>APAIQILNFTFDKSVITN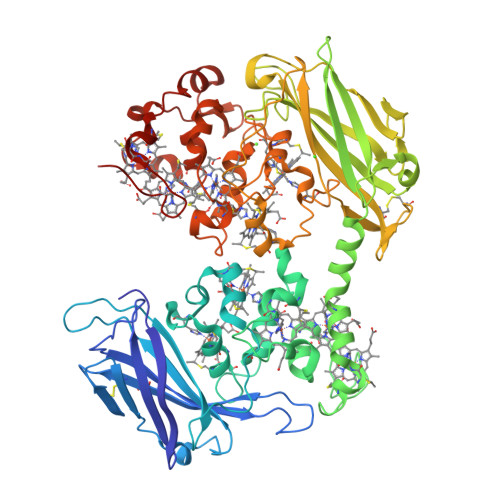GVPSVEFTVTNENDLPVVGLQKMRFAAAQLIPQGATGAGNASQWQYFGDETCDVAATCPGTFVDQKNGHYSYTFNMNLTANAKITYNDQLAQRVLIRAYNTPLPDGTQVPNSNAFVDFTADTGAAPTYSRKIVATESCNTCHQDLANVKHGGAYSDVNYCATCHTAGKVGVGKEFNVLVHAKHKDLTLGSLESCQSCHAANDAAPDWGNWSRIPTAATCGSCHSTVDFAAGKGHSQQLDNSNCIACHNSDWTAELHTGKTADKKAVIAQLGMQATLVGQTDDTAVLTVSILDKDGNAIDAATVQDKIKRLETVTNVGPNFPIMGYNKSPGSGAAKIAKDLVKDGALQAGVTLVDGKLVFTTPALPFGTGDTDTAFTFIGLEMCSTGTSLTACTVDSATTSMKAELAFGTKSGNAPSMRHVNSVNFSTCQGCHSDTFEIHKGHHSGFVMTEQVSHAKDANGKAIVGVDGCVACHTPDGTYASGANKGAFEMKLHVIHGEQGVIKECTQCHNDFNLDAFKVKGALATSAGKYTTPITATCTSCHAPESIGHGLENMGAIVNGDYVQANQAAQSETCFYCHKPTPTDHTQVKM[3x]Most diderm phyla from the Terrabacteria group have recently been shown to lack well-characterised OM attachment systems, but instead have OmpM, which could represent an ancestral tethering system in bacteria. OmpM consists of an N-terminal periplasmic S-layer homology (SLH) domain connected via a linker region to a C-terminal OM β-barrel. Here we use single particle cryo-EM, X-ray crystallography, molecular dynamics simulations, bioinformatic analyses and functional assays to show that OmpM1 from V. parvula (VpOmpM1) is a general porin with similar structural and functional properties to E. coli OmpF, with an additional mobile periplasmic region that can bind V. parvula PG and take on different folds.

Surprisingly, the crystallized stalk does not fold into a coiled-coil but forms a compact trimer composed mainly of α-helices (residues 23–105). The residues that form the coiled-coil in the extended AlphaFold2 prediction instead form helical hairpins and extensive intra-protomer interactions rather than interact with the other chains in the asymmetric unit. The protomer interfaces form grooves on one side of the trimer that could potentially accommodate ligands. However, mapping of the previously identified putative PG-binding residues onto the stalk crystal structure shows they are spread across the structure, suggesting that this conformation does not bind PG. The protomer fold of the stalk observed in the crystal structures aligns well with an alternative, compact conformation predicted by AlphaFold2. However, the trimerization interface in the compact stalk prediction is different: residues that are far away in the crystal structure (e.g., M75) interact in the predicted compact conformation. We considered that this compact state could be an unstable high energy conformation (hence the low prediction confidence), and that the stalk construct is stabilized in a similar conformation in the crystallization condition. Notably, the soluble SLH domain did not bind to V. parvula or E. coli sacculi, unlike the full-length VpOmpM1. This suggests that the structure of the isolated SLH domain is different than in the full-length protein, as observed by cryo-EM. Therefore, we do not believe that the conformation observed in the crystal structure is the result of crystal packing.

>MAANPFSDVTPDSWAYQAVSQLAQAGIVNGYPDGTFKGQNNITRYEMAQMVAKAMANQDRANAEQQAMINRLADEFSNELNNLGVRVSLEHHHHHH[3x]>[3x]GPDEEPEEPGRRGSFVEMVDNLRGKSGQGYYVEMTVGSPPQTLNILVDTGSSNFAVGAAPHPFLHR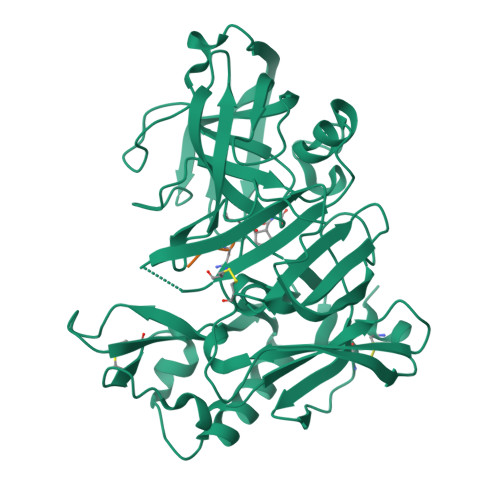YYQRQLSSTYRDLRKGVYVPYTQGKWEGELGTDLVSIPHGPNVTVRANIAAITESDKFFINGSNWEGILGLAYAEIARPDDSLEPFFDSLVKQTHVPNLFSLQLCGAGFPLNQSEVLASVGGSMIIGGIDHSLYTGSLWYTPIRREWYYEVIIVRVEINGQDLKMDCKEYNYDKSIVDSGTTNLRLPKKVFEAAVKSIKAASSTEKFPDGFWLGEQLVCWQAGTTPWNIFPVISLYLMGEVTNQSFRITILPQQYLRPVEDVATSQDDCYKFAISQSSTGTVMGAVIMEGFYVVFDRARKRIGFAVSACHVHDEFRTAAVEGPFVTLDMEDCGYNIPQTDES;>[3x]EVNXA> IVGGTASVRGEWPWQVTLHTTSPTQRHLCGGSIIGNQWILTAAHCFYGVESPKILRVYSGILNQSEIKEDTSFFGVQEIIIHDQYKMAESGYDIALLKLETTVNYTDSQRPISLPSKGDRNVIYTDCWVTGWGYRKLRDKIQNTLQKAKIPL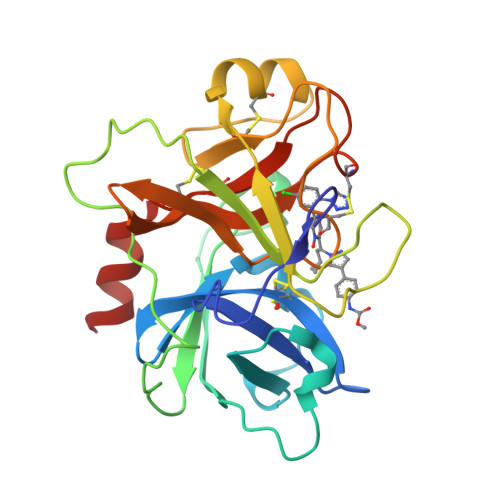VTNEECQKRYRGHKITHKMICAGYREGGKDACKGDSGGPLSCKHNEVWHLVGITSWGEGCAQRERPGVYTNVVEYVDWILEKTQAV> 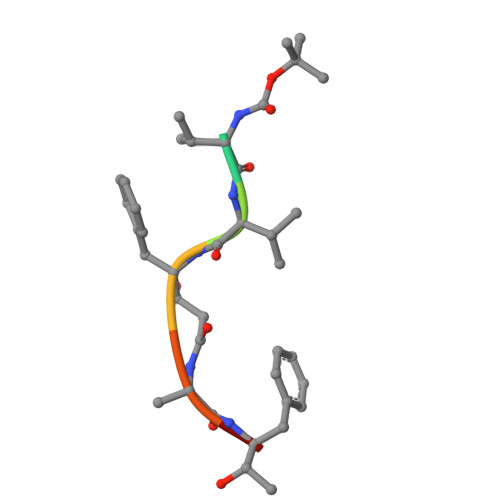XVVFAFA4-chloro-1H-benzimidazole | C7 H5 Cl N2 | 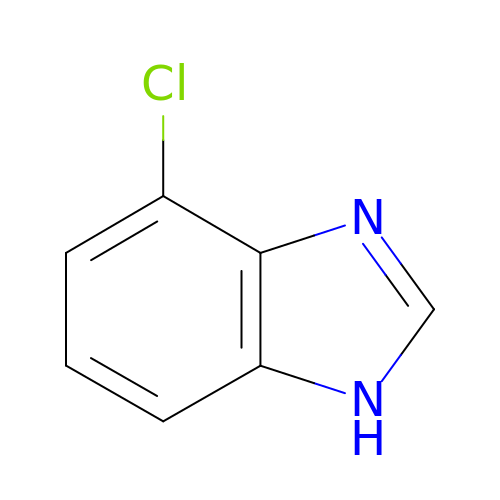RPYPMOKNVPZWKZ-UHFFFAOYSA-N>MDPMYLLVDVGNTHSVFSITEDGKTFRRWRLSTGVFQTEDELFSHLHPLLGDAMREIKGIGVASVVPTQNTVIERFSQKYFHISPIWVKAKNGCVKWNVKNPSEVGADRVANVVAFVKEYGKNGIIIDMGTATTVDLVVNGSYEGGAILPGFFMMVHSLFRGTAKLPLVEVKPADFVVGKDTE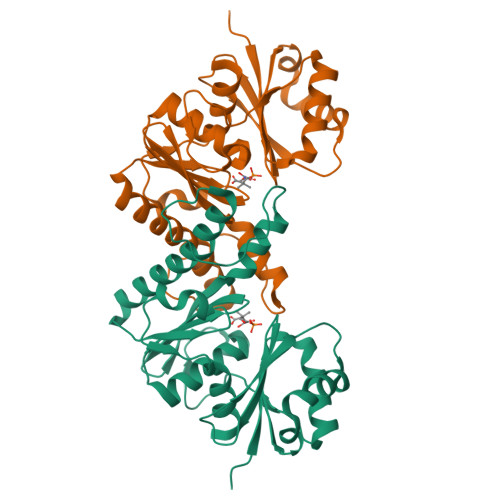ENIRLGVVNGSVYALEGIIGRIKEVYGDLPVVLTGGQSKIVKDMIKHEIFDEDLTIKGVYHFCFGD[6x]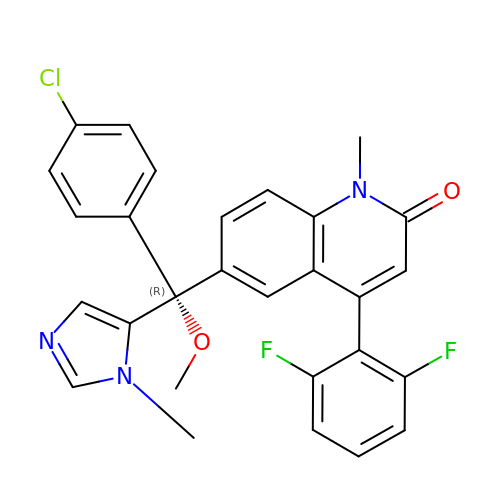6-[(R)-(4-chlorophenyl)(methoxy)(1-methyl-1H-imidazol-5-yl)methyl]-4-(2,6-difluorophenyl)-1-methylquinolin-2(1H)-one | C28 H22 Cl F2 N3 O2 | KVNUNQVIQXLHFU-MUUNZHRXSA-N>KTEMKDDFAKLEEQFDAKLGIFALDTGTNRTVTYRPDERFAFASTIKALTVGVLLQQKSIEDLNQRITYTRDDLVNYNPITEKHVDTGMTLKELADASLRYSDNTAQNLILKQIGGPESLKKELRKIGDEVTNPERFEPELNEVNPGETQDTSTARALATSLQAF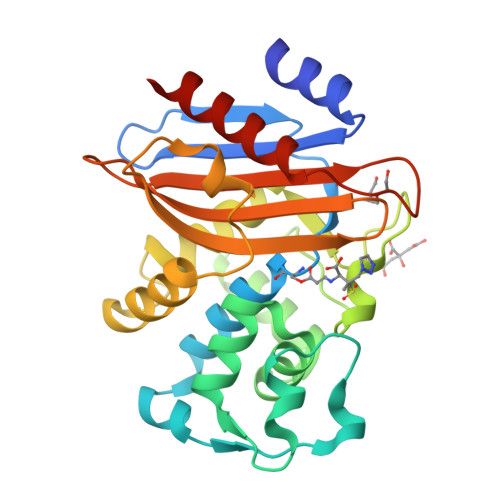ALEDKLPSEKRELLIDWMKRNTTGDALIRAGVPEGWEVADKTGAGSYGTRNDIAIIWPPKGDPVVLAVLSSRDKKDAKYDDKLIAEATKVVVKALNMNGK[2x]> YTRKMWSVQESEWLKQGVVRYGVGHWERIRSAFPFAGRTAVNLKDRWRTMVKLKM;> TRKMWSVQESEWLKQGVVRYGVGHWERIRSAF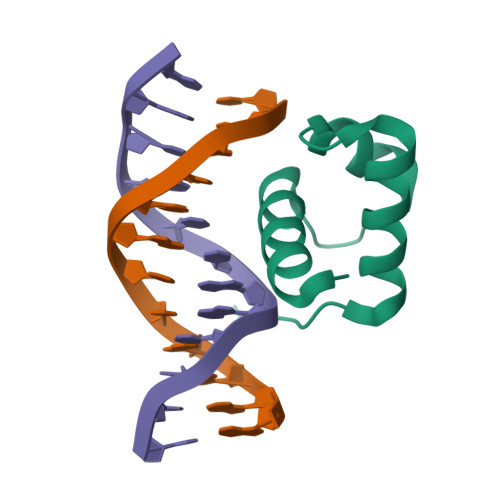PFAGRTAVNLKDRWRTMVKLKMV> MKIQMKTPLVELDGDEMTRVLWPLIKDKLLLPFIDLQTE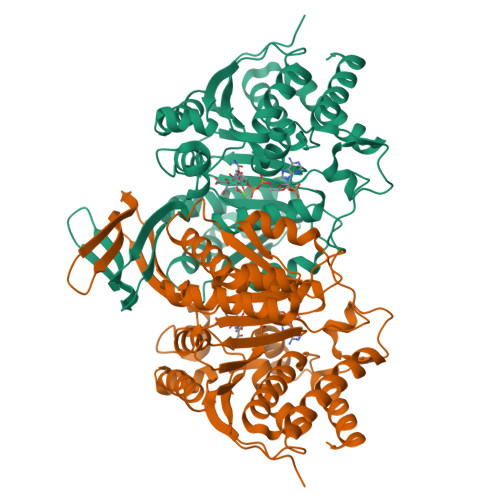YYDLGIEERDRTNDQITIDAAEAIKKYGVGVKNATITPNQDRVEEYGLKEQWKSPNATVRAMLDGTVFRKPIMVKNIKPSVRSWQKPIVVGRHAYGDFYKNAEIFAEAGGKLEIVVTDKNGKETRQTIMEVDEPAIVQGIHNTVASIGHFARACFEYSLDQKIDCWFATKDTISKQYDQRFKIIFEEIFAQEYKEKFAAAGIEYFYTLIDDVVARMMKTEGGMLWACKNYDGDVMSDMVASAFGSLAMMSSVLVSPYGYFEYEAAHGTVQRHYYQHLKGERTSTNPVALIYAWTGALRKRGELDGTPDLCAFCDSLEAITIECIESGYMTGDLARICEPAAIKVLDSIEFIDELGKRLQQLNK>[2x]SMSAPGYPFAKELCRIDAQNMGSRRMNVNNDLHPYISCNISDFKAQKFLINVSDTGLYIKTKYQDREMFPFLSQIEMARAAGAMASGNPIIKLTELSFREPMLQSGSNEQIRIVLTPDNQGASYSIEKQSDSSIYSSGRLELEGGAYENGNIHLEPFLSQRADRIPHEAFYQRLAEFGYSCSDSLKAAEHCVSR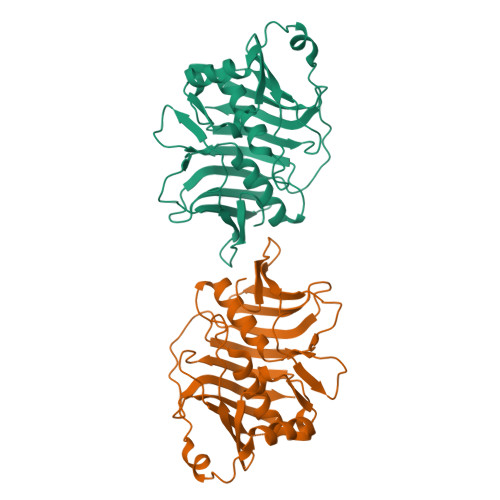NGQVLLKIKAKAGPKGCIIKPEVIESVYQAVIYLAGENAGELPENIKECTIFDHETEPVYVYAEQTGESDSAYDVYVLDNAGGILMELSGLVFGEKPNKNVRFYEHKWNQKNPLIEIK>[3x]MELNNVILEKEGKVAVVTINRPKALNALNSDTLKEMDYVIGEIENDSEVLAVILTGAGEKSFVAGADISEMKEMNTIEGRKFGILGNKVFRRLELLEKPVIAAVNGFALGGGCEIAMSCDIRIASSNARFGQPEVGLGITPGFGGTQRLSRLVGMGMAKQLIFTAQNIKADEALRIGLVNKVVEPSELMNTA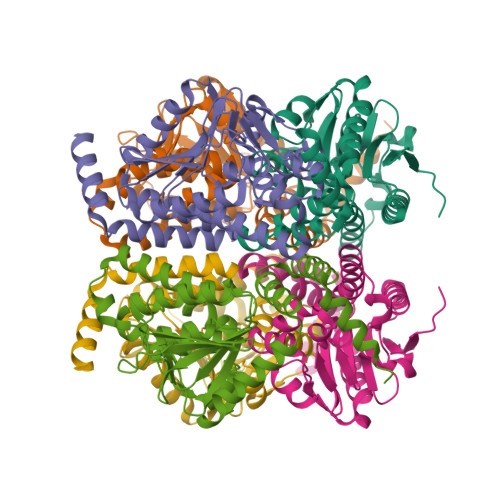KEIANKIVSNAPVAVKLSKQAINRGMQCDIDTALAFESEAFGECFSTEDQKDAMTAFIEKRKIEGFKNRHHHHHH>[4x]SLPHQPIPPSLGEKDLSDPFNFLFSSNKITLRKLYDLTKNVDFDQLRQNECKKNITLSKFWEKSEQRNVPEDDNWERFYSNIGSCSVYSDDQMIDNLLHDLNTSPIKHVHIMDGGTQ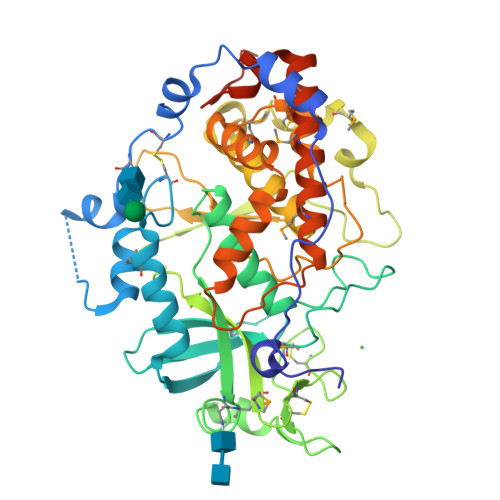VKFVFTFKNDKQAVFKPMRFGRDYESDPNHFYFSDFERHHAEIATFHLDRVLGFRRAIPTVGRVLNMTTELFEKAEKKLKKTFFFSPAKNFCFVSRCDYYCDTTHAICGLPDMKEGSVQVFLPDESAVPRKHNRSPYRRTYSKKNQVAEWQSSMNYCTDKVKTKRQYAHGRRLLDLVDIHILDYLIGNQDRHHFESFNVFNDLPSYAIHLDHGRAFGRSDFDDDDIILPLRQCCILRPSTFQTLMNFYSTPKSLTKALHESLSKDPAHPILAYKHYPAMERRLAKIMSHILECFESRGVAEVLVAEYNNPDVSDAEQNDEEQSEEHQDKKDDKKTV Two mammalian homologs of systemic RNA interference defective protein 1 (SID-1) (SIDT1/2) are suggested to function as double-stranded RNA (dsRNA) transporters for extracellular dsRNA uptake or for release of incorporated dsRNA from lysosome to cytoplasm. Here, we determine the cryo-electron microscopy structures of human SIDT1, homodimer in a side-by-side arrangement, with two distinct conformations, the cholesterol-bound form and the unbound form. Our structures reveal that the membrane-spanning region of SIDT1 harbors conserved histidine and aspartate residues coordinating to putative zinc ion, in a structurally similar manner to alkaline ceramidases or adiponectin receptors that require zinc for ceramidase activity. We identify that SIDT1 has a ceramidase activity that is attenuated by cholesterol binding.

SIDT1 embedded in a GDN micelle exhibited the 2D averages of relatively resolved transmembrane helices and we successfully generated a reconstruction of hSIDT1 to an overall resolution of 2.77 Å. The lipid-like densities were inserted at the cytoplasmic side of TM region. These densities were fitted to cholesterol molecules and Mass spectrometry analysis identified cholesterol in purified hSIDT1. The two densities run parallel to each other in a small concave formed by TM5, TM6, and TM7 at the intracellular side, which can be modeled as cholesterol molecules. The putative cholesterol density which is better resolved than the other (CLR1) is located on the opposite of the homo-dimer interface of TM5 and fills the space between TM5 and TM6. Another cholesterol molecule (CLR2) is packed with TM5 and TM7. These cholesterol molecules were surrounded by hydrophobic residues, most of which are conserved in mammalian SID-1 family proteins, suggesting that the cholesterols serve as molecular glue that stabilizes the conformation of TM5, TM6, and TM7.SIDT1 is previously reported to bind cholesterol via CRAC motif16 characterized by the sequence (L/V)-X1−5-(Y)-X1−5-(K/R)25. On the extracellular side of the TM helices, we detected density that would be assignable to Zn2+, being tetrahedrally coordinated with His563, Asp574, His791 and His795. In the cholesterol-bound form of SIDT1, Zn2+ is coordinated by the conserved three His residues and Asp residue, in which there is no space for a water molecule which is activated through the coordination with Zn2+.

>[2x]MRGCLRLALLCALPWLLLAASPGHPAKSPRQPPAPRRDPFDAARGADFDHVYSGVVNLSTENIYSFNYTSQPDQVTAVRVYVNSSSENLNYPVLVVVRQQKEVLSWQVPLLFQGLYQRSYNYQEVSRTLCPSEATNETGPLQQLIFVDVASMAPLGAQYKLLVTKLKHFQLRTNVAFHFTASPSQPQYFLYKFPKDVDSVIIKVVSEMAYPCSVVSVQNIMCPVYDLDHNVEFNGVYQSMTKKAAITLQKKDFPGEQFFVVFVIKPEDYACGGSFFIQEKENQTWNLQRKKNLEVTIVPSIKESVYVKSSLFSVFIFLSFYLGCLLVGFVHYLRFQRKSIDGSFGSNDGSGNMVASHPIAASTPEGSNYGTIDESSSSPGRQMSSSDGGPPGQSDTDSSVEESDFDTMPDIESDKNIIRTKMFLYLSDLSRKDRRIVSKKYKIYFWNIITIAVFYALPVIQLVITYQTVVNVTGNQDICYYNFLCAHPLGVLSAFNNILSNLGHVLLGFLFLLIVLRRDILHRRALEAKDIFAVEYGIPKHFGLFYAMGIALMMEGVLSACYHVCPNYSNFQFDTSFMYMIAGLCMLKLYQTRHPDINASAYSAYASFAVVIMVTVLGVVFGKNDVWFWVIFSAIHVLASLALSTQIYYMGRFKIDLGIFRRAAMVFYTDCIQQCSRPLYMDRMVLLVVGNLVNWSFALFGLIYRPRDFASYMLGIFICNLLLYLAFYIIMKLRSSEKVLPVPLFCIVATAVMWAAALYFFFQNLSSWEGTPAESREKNRECILLDFFDDHDIWHFLSATALFFSFLVLLTLDDDLDVVRRDQIPVFENLYFQGDYKDDDDKHHHHHHHH>[3x]MGSSHHHHHHSAALEVLFQGPDYKFWYTQPVPKINDEFNESVNEPFISDNKVEDVRKDEYKLPPGYSWYVCDVKDEKDRSEIYTLLTDNYVEDDDNIFRFNYSAEFLLWALTSPNYLKTWHIGVKYDASNKLIGFISAIPTDICIHKRTIK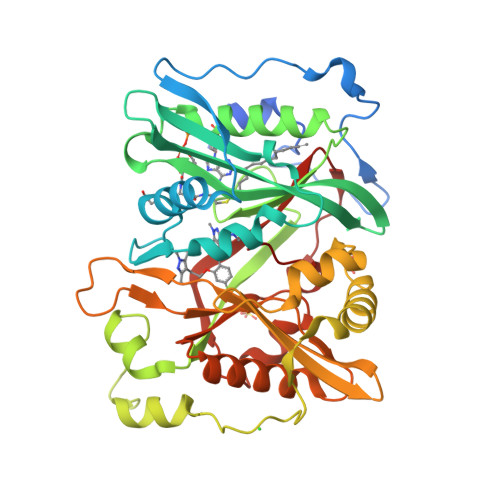MAEVNFLCVHKTLRSKRLAPVLIKEITRRINLENIWQAIYTAGVYLPKPVSDARYYHRSINVKKLIEIGFSSLNSRLTMSRAIKLYRVEDTLNIKNMRLMKKKDVEGVHKLLGSYLEQFNLYAVFTKEEIAHWFLPIENVIYTYVNEENGKIKDMISFYSLPSQILGNDKYSTLNAAYSFYNVTTTATFKQLMQDAILLAKRNNFDVFNALEVMQNKSVFEDLKFGEGDGSLKYYLYNWKCASFAPAHVGIVLL Human dipeptidyl peptidase III (hDPP III), also known as enkephalinase B, is a member of the M49 family of zinc dependent metallopeptidases and cleaves dipeptides sequentially from the N-terminus of various bioactive peptide substrates. Crystal structures have so far been determined for DPP III from humans as well as from Saccharomyces cerevisiae. Despite the low sequence identity (36%) shared by the two proteins, both structures are very similar and consist of two lobes separated by a wide cleft. The “upper” lobe is mostly α-helical and contains the zinc binding site as well as the catalytically important residues. In both structures, two histidine residues (His-450 and His-455 in the human enzyme) and a glutamate (Glu-508) coordinate the zinc ion.

Met-enkephalin (YGGFM) and Leu-enkephalin (YGGFL) are endogenous opioid neurotransmitters which are found in the brains and spinal cords of many animals, including humans, and which have been shown to be cleaved by hDPP III1. In the complex structures, the N-termini of both peptides are anchored to the protein through hydrogen bonding and electrostatic interactions from the side chains of Tyr-318, Glu-316 and Asn-394. The first three amino acids form a β-strand, which interacts with the five-stranded β-core in an antiparallel fashion (through hydrogen bonds to Ala-388 to Asn-391). These interactions stabilize the extended conformation of the peptide, which would otherwise not be favoured due to the glycine residues at positions 2 and 3 of the enkephalins. One exception is His-568 from the upper lobe, which is hydrogen bonded to the carbonyl oxygen of the scissile peptide bond. Quite unexpectedly, the zinc ion does not directly interact with the P1 carbonyl of the peptide (the scissile peptide) but is at a distance of 3.7 Å and 3.6 Å for Met and Leu-enkephalin, respectively. Instead, a water molecule completes the tetrahedral coordination of the metal ion. In the complex with Met-enkephalin the zinc bound water molecule is situated right between the side chain of Glu-451 and the scissile amide bond. Despite the uncertainties regarding the exact conformation of Glu-451, this configuration can be considered structurally similar to the Michaelis complex and the water molecule is in a suitable position for the nucleophilic attack on the peptide group. In the case of efficiently cleaved peptides like the enkephalins, on the other hand, the reaction follows the energetically favoured and therefore faster water mediated hydrolysis pathway.

> MADTQYILPNDIGVSSLDSREAFRLLSPTERLYAYHLSRAAWYGGLAVLLQTSPEAPYIYALLSRLFRAQDPDQLRQHALAEGLTEEEYQAFLVYAAGVYSNMGNYKSFGDTKFVPNLPKEKLERVILGSEAAQQHPEEVRGLWQTCGELMFSLEPRLRHLGLGKEGITTYFSGNCTMEDAKLAQDFLDSQNLSAYNTRLFKEVDGCGKPYYEVRLASVLGSEPSLDSEVTSKLKSYEFRGSPFQVTRGDYAPILQKVVEQLEKAKAYAANSHQGQMLAQYIESFTQGSIEAHKRGSRFWIQDKGPIVESYIGFIESYRDPFGSRGEFEGFVAVVNKAMSAKFERLVASAEQLLKELPWPPTFEKDKFLTPDFTSLDVLTFAGSGIPAGINIPNYDDLRQTEGFKNVSLGNVLAVAYATQREKLTFLEEDDKDLYILWKGPSFDVQVGLHALLGHGSGKLFVQDEKGAFNFDQETVINPETGEQIQSWYRCGETWDSKFSTIASSYEECRAESVGLYLSLHPQVLEIFGFEGADAEDVIYVNWLNMVRAGLLALEFYTPEAFNWRQAHMQARFVILRVLLEAGEGLVTITPTTGSDGRPDARVRLDRSKIRSVGKPALERFLRRLQVLKSTGDVAGGRALYEGYATVTDAPPESFLTLRDTVLLRKESRKLIVQPNTRLEGSDVQLLEYEASAAGLIRSFSERFPEDGPELEEILTQLATADARFW;> YGGFM>[6x]PECVVDAGKVTLGTQQRQEMDPRLREKQNEIILRAVCALLNSGGGIIKAEIENKGYNYERHGVGLDVPPIFRSHLDKMQKENHFLIFVKSWNTEAGVPLATLCSNLYHRERTSTDVMDSQEALAFLKCRTQTPTNINVSNSLGPQAAQGSVQYEGNINVSAAALFDRKRLQYLEKLNLPESTHVEFVMFSTDVSHCVKDRLPKCVSAFANT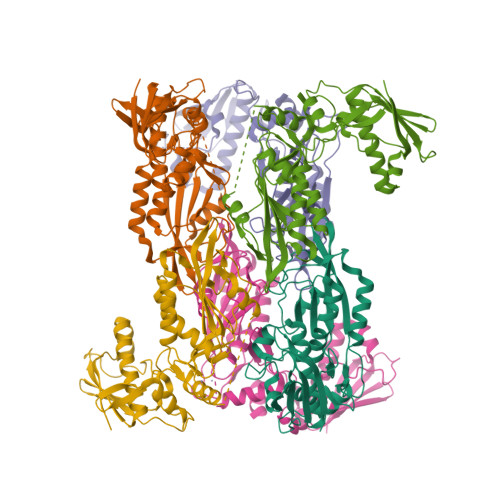EGGYVFFGVHDETCQVIGCEKEKIDLTSLRASIDGCIKKLPVHHFCTQRPEIKYVLNFLEVHDKGALRGYVCAIKVEKFCCAVFAKVPSSWQVKDNRVRQLPTREWTAWMMEADP Virus ΦcrAss001 (Kehishuvirus primarius) was the first representative of this order to be isolated in pure culture from human faecal samples. Here, we present the characterization of ΦcrAss001 using cryo-electron microscopy (cryo-EM), enabling de novo structure building and elucidation of functions for around 1,440 protein subunits constituting the virion, leading to the identification of a novel ‘crass fold’ in the distal part of the tail. The virion possesses a short non-contractile tail extending approximately 44 nm from an icosahedral capsid. The extended tail barrel formed by widely conserved paralogous ring proteins has a high capacity for storage of cargo proteins alongside the capsid cargo zone, ensuring that the proteins required for the initial stages of crassvirus infection are carried inside virions and delivered to the host cell.

The icosahedral reconstruction of the capsid, which was determined to a resolution of 3.01 Å, has an outer diameter of approximately 88 nm. The capsid has a triangulation number (T) of nine, with an asymmetric unit comprising nine copies of the major capsid protein (MCP) gp32, nine copies of the capsid auxiliary protein gp36, one copy of the trimeric head fibre protein (HFT) gp21, and two copies of the dimeric head fibre protein (HFD) gp29. The MCP adopts the HK97-like fold—the canonical fold of the capsid proteins of the viruses in the class Caudovirecetes14, with the main body comprising the A-domain and P-domain. A β-barrel insertion in the E-loop, composed of residues 79–180 (I-domain), is a widespread feature of the crassviruses. This insertion domain forms a three-fold symmetric assembly with the auxiliary protein at the capsid surface, making up much of the exposed surface of the capsid and contributing substantially to the capsid wall thickness and stability. The FD domain of the auxiliary protein interacts with the A-domain of the MCP, around the periphery of each hexamer and pentamer. Each hexamer can adopt one of two conformations: winged or planar. Winged hexons span the edges of the icosahedron, on both sides of the icosahedral two-fold symmetry axes, whereas planar hexons are positioned at the three-fold symmetry axes. At the centre of each hexon is a pocket formed by the MCP and auxiliary protein, which serves as a binding site for fibre proteins. A trimer of the head fibre protein gp21 (residues 1–38) binds in the planar hexon pocket at the three-fold symmetric site, whereas a dimer of the capsid fibre protein gp29 (residues 1–58) binds in the winged hexon.

>[9x]MAGKLGKFQMLGFQHWKGLTSDNHLGAIFQQAPQKATNLMVQLLAFYRGKSLDTFLNSFPTREFEDDNEYYWDVIGSSRRNIPLVEARDENGVVVAANAANVGVGTSPFYLVFPEDWFADGEVIVGNLNQVYPFRILGDARMEGTNAVYKVELMGGNTQGVPAERLQQGERFSIEFAPVEKELSRKVGDVRFTSPVSMRNEWTTIRIQHKVAGNKLNKKLAMGIPMVRNLESGKQVKDTANMWMHYVDWEVELQFDEYKNNAMAWGTSNRNLNGEYMNFGKSGNAIKTGAGIFEQTEVANTMYYNTFSLKLLEDALYELSASKLAMDDRLFVIKTGERGAIQFHKEVLKTVSGWTTFVLDNNSTRVVEKVQSRLHSNALSAGFQFVEYKAPNGVRVRLDVDPFYDDPVRNKILHPMGGVAFSYRYDIWYIGTMDQPNIFKCKIKGDNEYRGYQWGIRNPFTGQKGNPYMSFDEDSAVIHRMATLGVCVLDPTRTMSLIPAILQG;>[9x]MVISINQVRQLYVAKALKANTAALTTAGDIVPKADTAKTTLYFQSMSPAGIVASDKINLKHVLYAKATPSEALAHKLVRYSVTLDADVSATPVAGQNYILRLAFRQYIGLSEEDQYFKYGEVIARSGMTASDFYKKMAISLAKNLENKTESTPLVNIYLISAAAASTDVPVTSATKESDLTATDYNQIIIEETEQPWVLGMMPQAFIPFTPQFLTITVDGEDRLWGVATVVTPTKTVPDGHLIADLEYFCMGARGDIYRGMGYPNIIKTTYLVDPGAVYDVLDIHYFYTGSNESVQKSEKTITLVAVDDGSHTAMNALIGAINTASGLTIATL;>[2x]MKRVLNLGNLSRIVEGDPNEITDDEILVIKDKIIEGKIIDIQKRVDGKLVSLITEKYTYTINPTPADAIVVINGSTTKSIRAAKGHTVTWSVSKTGFVTQSGSDVISGDVSKDVTLVANPAS;> MKTLRTLKISPNAPDINSVWLYKGTMKYFNNGEWETIGGESEPYVLPAATTSTIGGVKKATNVGNLATGAELATVVTKVNAILSALKVADIMVEDAN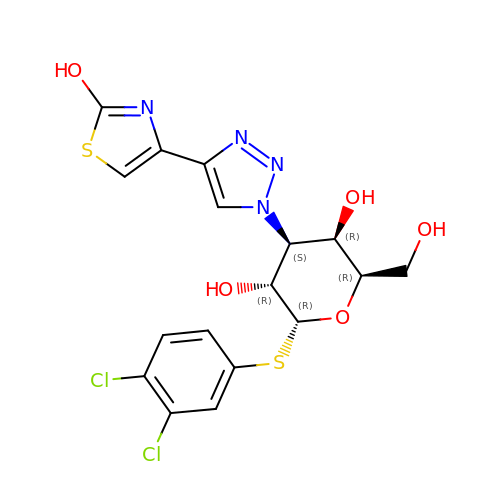(2~{R},3~{R},4~{S},5~{R},6~{R})-2-(3,4-dichlorophenyl)sulfanyl-6-(hydroxymethyl)-4-[4-(2-oxidanyl-1,3-thiazol-4-yl)-1,2,3-triazol-1-yl]oxane-3,5-diol | C17 H16 Cl2 N4 O5 S2 | BWEZCWXAMQJAHD-LYYZXLFJSA-N>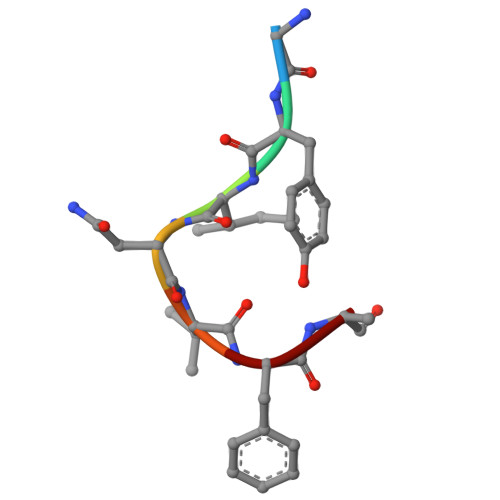 GYINVFA> YEYYNELAENKTYKKLAIEAPRGEIKDRYGRLLAGNKNLFTVQVSGNDINKKDANKHSRANEISLKLINLLERNGEEYVDEFPIYVENGKYYYTYDRDIREYKSENGIPNDYNAKESFYYLVDKLISAGILSQEDKRLDATRLQAKLNENGYYPPILVSKWMFTAERDKRDWLASYKIKETKLSAKEAFEKVRNSDALEIDKSLSDEDARKIMVVRDLIKSKGYSQYNPVTIAKDVGETTIAQIEESAMDLVGVSIAVEPVRYYPNGSLASHMLGYVGKMPSTQIESYLQKGYETGDMVGLAGVEKSNESRLRGTDGYKMVKVDALGRISKEIESKKPKSGDTVYLTLDKDLQEVSDNALKQIIEVASKGGTFKSKFGDKPISAYAGKAQSAALIAIDVKNGEVLASSSYPNYDPNKFAKGISTEDYKALQPKNPNDLLAGSPLLNLVTQGEFQPGSSFKMLTSMAALENGLDPNFTINDPGVIMLGKKSFGDYVWNHGRGNHGMTNLYKAIQESCNIYMATIGTGKTWPDGKSIGIDMNANKILEYAKLFGLDQNTGLQDEVEERAGKVPSTEDKLKSTQALLKSNLERE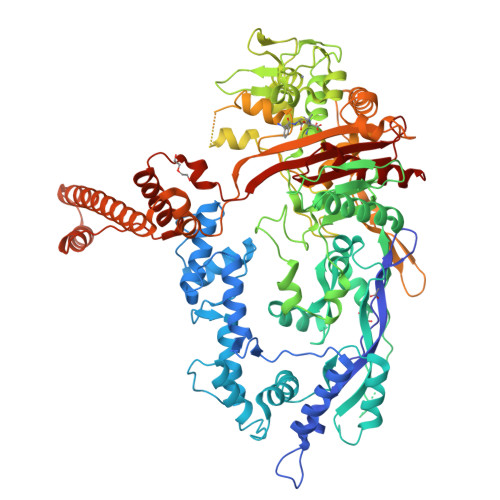MANDFVDITREKNPKEYEKRINEIVSWAAEKKTPGRVETMNRLKKMNVKEDRIEEVADLAVFSYFNFAKWSTADTFNLAIGQGENAYTPAQISRYVAAIANGGNLVELSVVDRAVSSDYSSVKINDQKKVEKIPFKNPDNLKELTKGMKLVARQGTAKSAFADFPIDVAAKTGTAEKSGKIPTDNEYEYLKSHMSSYNVNLNDAIKLADKMKAEKEKELSLAKEKEIKKKLENKDLKDEERKKLEEELEDGVKVRLEDTDKVNSSYLRKAIKELNPKITDDQIDRFKQDYGSFTWTVAFAPADDPEIAVVCVIPQGDSSVFSLLPTREVIGTYMGL>FRKTIDQKKPCKHFSFYFHDILYDGDNVANATSAAIVSPPGLGNFKFGKFVIFDGPITMDKNYLSKPVARAQGFYFYDMKMDFNSWFSYTLVFNSTEHKGT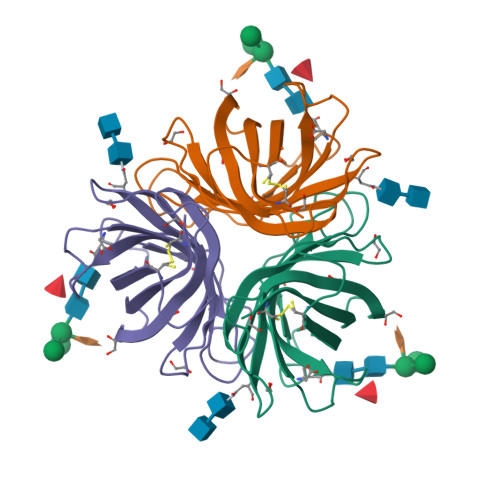LNIMGADLMMEPTRDLSVVGGTGDFFMARGIATFVTDLFQGAKYFRVKMDIKLYECY[2x]[(R)-(2,4-dichlorophenyl)(sulfanyl)methyl]phosphonic acid | C7 H7 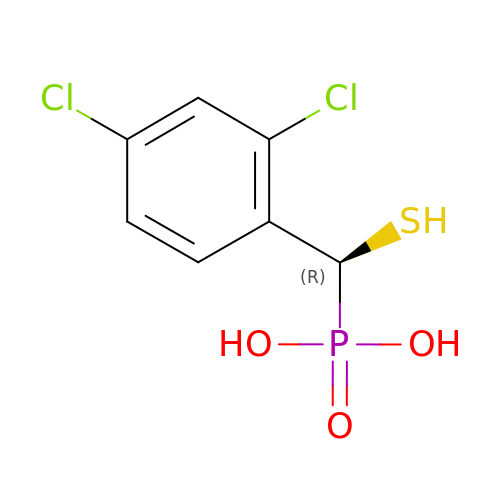Cl2 O3 P S | WJVBVZOYOCLGPI-SSDOTTSWSA-N> MGDTKEQRILRYVQQNAKPGDPQSVLEAIDTYCTQKEWAMNVGDAKGQIMDAVIREYSPSLVLELGAYCGYSAVRMARLLQPGARLLTMEMNPDYAAITQQMLNFAGLQDKVTILNGASQDLIPQLKKKYDVDTLDMVFLDHWKDRYLPDTLLLEKCGLLRKGTVLLADNVI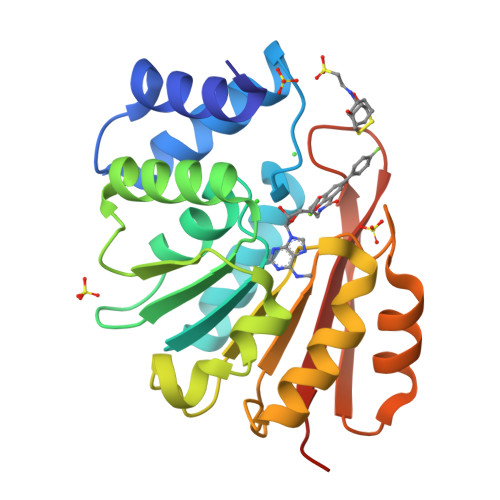VPGTPDFLAYVRGSSSFECTHYSSYLEYMKVVDGLEKAIYQGPSSPDKS> MVVKRTQTDSRMQSTPGNHNHPDAHANAAYMTPPSMGALNANNSNSQLSTLTISPMTYLANNTSTDGSFLKERNAQNTDSLSREDYLRLWRHDALMQQQYKCAAFVGEKVLDITGNPNDAFWLAQVYCCTGDYARAKCLLTKEDLYNRSSACRYLAAFCLVKLYDWQGALNLLGETNPFRKDEKNANKLLMQDGGIKLEASMCYLRGQVYTNLSNFDRAKECYKEALMVDAKCYEAFDQLVSNHLLTADEEWDLVLKLNYSTYSKEDAAFLRSLYMLKLNKTSHEDELRRAEDYLSSINGLEKSSDLLLCKADTLFVRSRFIDVLAITTKILEIDPYNLDVYPLHLASLHESGEKNKLYLISNDLVDRHPEKAVTWLAVGIYYLCVNKISEARRYFSKSSTMDPQFGPAWIGFAHSFAIEGEHDQAISAYTTAARLFQGTHLPYLFLGMQHMQLGNILLANEYLQSSYALFQ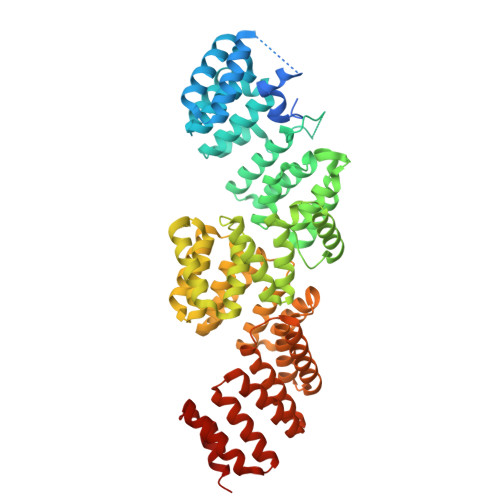YDPLLLNELGVVAFNKSDMQTAINHFQNALLLVKKTQSNEKPWAATWANLGHAYRKLKMYDAAIDALNQGLLLSTNDANVHTAIALVYLHKKIPGLAITHLHESLAISPNEIMASDLLKRALEEN> GAMGGFPNDAKGISGNGKYYSLGQIEKLYSNQFATYNNLTVITSDTHENSDNFAFCLANGKRFPSFTDEKPKGIYTLVKDINKEQYTKLLKENHKWSSIPNLNQAWDTFSRLSYMYLKDPTDIVKRAWGTDLNTARTYFHQVIQYEIWRYTDGMRVSSDTNVYIYEKFSPQQKKALEMIRTDLYNFTVPYENLEYRFYKPDWVFG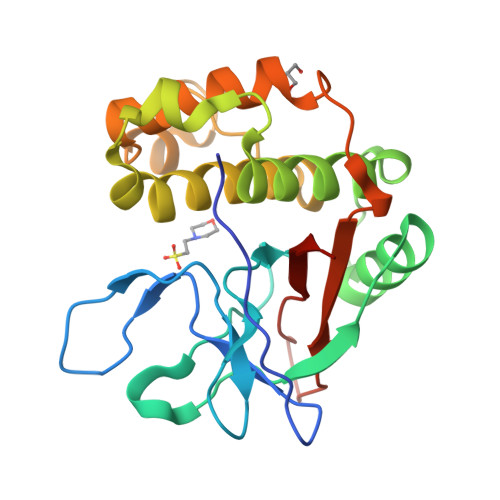LGFQALATVRWKIEP>MNTKTRLTNDSQQQIDKIIEHDLQKGHIPGASILIVKNGKVFLNKGYG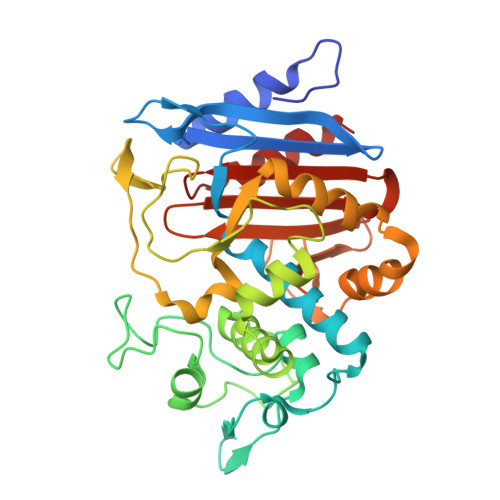YQDVDKKVKASPTTKYEIASNTKAFTGLAILKLAQEGRLNLNDDVSKHVPHFKMNYNGQNETITIKQLLAQTSGIPSDITSEDAVTNKNNRLNDVTRAIMGDELHHKPGEEFEYSNMNYDLLGLIIQNVTKQSYTKYITNSWLKPLHMTHTSFKQTNNKSKHDAIGYELQGSTPVVSKPEFNLWDTPSAYMMTSTEDLEHWIKFQLNPPDKYKSLVQQSHKNLSSTIGEPNANAYASGWFTNNDEHLVFHSGTLDNFSSFILLNPKQNYGIVVLANLNSEYVPKLVEHLNTQIV[4x]>[2x]GSHMAGNDSNLIWLDLEMTGLEPVEDVILEIAIIITDSELNILAQGPIFAISQTDDVLDNMNPWCIEHHGKSGLTQRCRDSEVSLAHATKESLAFVQEWVPQGKSPMCGNSIGQDRRFINKYMPDFEDHFHYRNLDVSTIKELAKRWKPEVLESVVKTGAHLALDAIKESIAELKVYRELFFKL

Therefore, oligoribonucleases (ORN), RNases targeted toward short oligonucleotides, are needed for the complete digestion of short oligonucleotides into mononucleotides. Among these, ORN belongs to the DEDD superfamily, comprising 3′-5′ exonucleases that require a divalent cation for activity. Our research group have focused on the mechanism of action of oligoribonuclease (CpsORN) from the psychrophilic gram-negative bacterium Colwellia psychrerythraea strain 34H, to understand how the enzyme hydrolyses small nucleic acids. Structural analysis results show that CpsORN is a stable dimer and its active site is formed by swapping residues from the other subunit.

The putative active site of CpsORN was confirmed by solving the structure of the pNP-TMP-bound CpsORN (D163A inactive mutant). The pNP-TMP complexed D163A mutant CpsORN crystal contains two pNP-TMP molecules in the active site of each monomer, but no metal ion was found at the expected position of the magnesium ion. This is consistent with the fact that the D163A mutant has no RNase activity, and bound pNP-TMP is not cleaved in pNP-TMP complexed CpsORN structure. Structural alignment between the unliganded form and the pNP-TMP-bound D163A mutant structure of CpsORN has 0.503 Å overall r.m.s deviation for 159 Cα atoms. The major structural differences were found in the α2 helix and the α8-α9 loop region near the active site, suggesting that ligand-binding induces these conformational changes. Detailed examination revealed that the side chain of Trp61, located on the α2 helix is flipped, and extends to the active site. This change leads to the shift of the α2 helix toward the active site. The α8-α9 loop region also shifts slightly toward the active site and interacts with the bound pNP-TMP. These conformational changes generate the closed state of pNP-TMP-bound CpsORN compared to the unliganded form of CpsORN.> SIKTPEDIEKMRVAGRLAAEVLEMIEPYVKPGVSTGELDRICNDYIVNEQHAVSACLGYHGYPKSVCISINEVVCHGIPDDAKLLKDGDIVNIDVTVIKDGFHGDTSKMFIVGKPTIMGERLCRITQESLYLALRMVKPGINLREIGAAIQKFVEAEGFSVVREYCGHGIGRGFHEEPQVLHYDSRETNVVLKPGMTFTIEPMVNAGKKEIRTMKDGWTVKTKDRSLSAQYEHTIVVTDNGC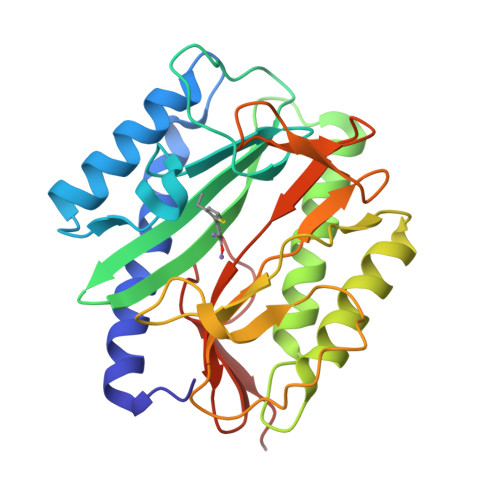EILTLRKDDTIPAIISHDE>[2x]NKLSGLIAAPHTPFAADGSVNYPVIDDIAKHLIATGVTGAYVLGTTGEGIHCSVEERKKVAERWVTASQGQLDLIIHTGALSIADTLELARHAE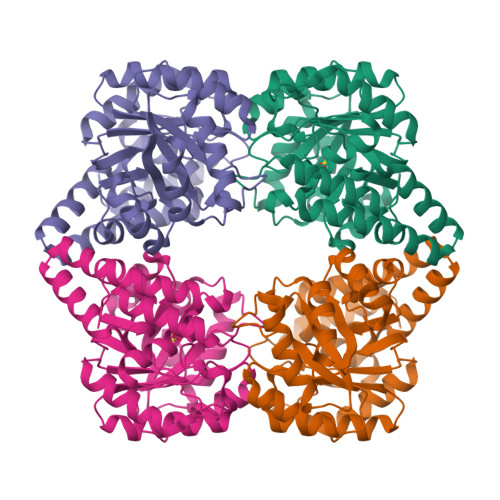TLDIKATSVIGPCFFKPSHVDDLVEYCRLAAASAPSKGFYYYHSTMSGLSIDMEKFLQAAGKVIPNLSGMKFNSPDMYEFQRCLRVEGGKYDIPFGVDEFIPAGLACGALSAVGSTYNYAAPLYLELIEKFNQGDHQGVADCMDKVIAIIRVLVEYGGVAAGKVAMQLHGIDVGAPRRPLRPLTAEQKADALAKFKAANFL To date, family GH139 is the only family known to be able to degrade α1,2-linked MeFuc, making it essential for RG-II metabolism and a feature of RG-II-degrading bacteria. In this report, we present the 3D structure of BT0984GH139, alongside its homolog SDT91673.1GH139 from Verrucomicrobium sp. GAS474, an organism isolated from forest soil. Crystals of BT0984GH139 formed in space group P212121 and diffracted to a resolution of 2.7 Å, while crystals of SDT91673.1GH139 formed in space group P 6522 and diffracted to 2.05 Å, providing good quality electron density maps in both cases. Both proteins adopt a three-domain architecture, consisting of an N-terminal β-sheet domain leading into an α-helical domain composed of a core (α/α)6 toroid structure. GH139 enzymes operate via an inverting mechanism in which we propose that N412 functions as the catalytic base and E561 acts as the catalytic acid (BT0984GH139 numbering).

The B. theta protein BT0984 was the founding member of GH139 (BT0984GH139) and is specific for the α1,2-linked MeFuc in chain B(6). BT0984GH139 specifically cleaves α1,2 linked MeFuc in partially digested RG-II but cannot access this residue within the intact polysaccharide. However, once the preceding arabinofuranose (Araf) and rhamnose (Rha) residues have been removed, BT0984GH139 can efficiently remove MeFuc from isolated chain B. BT0984GH139 exhibited no activity on 4-nitrophenyl α-L-fucoside (4NP-Fuc) but displayed activity on 4-nitrophenyl 2-O-methyl-α-L-fucoside (4NP-MeFuc). By 3 h the anomeric signals had reached equilibrium. These data indicate BT0984GH139 produces β-MeFuc and performs cleavage with inversion of the anomeric configuration of the α-MeFuc linkage. In BT0984GH139, a triad of Trp residues, W162, W403, and W490, lines the putative positively numbered subsites, providing aromatic stacking interactions for sugars within the Δbt0984 oligo. D723 forms hydrogen bonds with both N412 and N729, at distances of 3.3 Å and 2.9 Å, respectively, suggesting it may fulfill the role of activating N412 to function as a catalytic base. In BT0984GH139, the amide side chain of Q411 is positioned 3.5 Å from the catalytic acid E561, and could fulfill the same role as N421 in AfcAGH95 upon substrate binding. Surprisingly, overnight endpoint assays revealed that only one mutation in BT0984GH139, E561A, completely inactivated the enzyme. Based on these data, and with comparison to GH95, it appears that N412 and E561 function as the catalytic base and acid, respectively, in an inverting catalytic mechanism.

>[2x]MGSSHHHHHHSSGPQQGLRQHANVVWDTPSRNSSESMPCGGGDIGMNIWVEEGDILFYLSRSGTFDENNCQLKQGRFRLRLSPNPFEDAKDFRQELKLIDGYVEISAEGTQVQLWADVFHPVVHIEVINDRPLQAEIFYENWRYQDRLIRKGEGQQCSYKWAPPKGTMTHADFISLENSSEKDSKRLLFYHRNAEETVFDVAVAQQGMNEVKSQMMNPLKNLTFGGYLSGENLEYIGTSDSVYAGTDYRAWGFRSLKASKKHHFSVVLHTEQTETVTQWEQGLKTAWQRIAPQGKISSKVVSQDKKQTRLWWNAFWQRSFIETIGETENKENSKVEKETGNKEKSDAKDALKEITRNYTLFRYMLGCNAYGSVPTKFNGGLFTFDPCHIDEKQAFTPDYRKWGGGTMTAQNQRLVYWPMLKSGDFDMMPSQFNFYNRMLKNAELRSHVYWQHEGACFCEQIENFGLPNPAEYGFKRPAWFDKGLEYNAWLEYEWDTILEFCQMILETKNYAGADITPYLPLIESSLTFFDEHYRLLASRRGRKALDGDGHLILFPGSACETYKMTNNASSTIAALRTVLETYIKVCNNEKWQKMLETIPPVPLRYIEVKDSLNLQASTMTPAWKQTISPAKSWERINNIETPQLYPVFPWRIYGVGKENLEIARDTYFYDPDALKFRSHTGWKQDNIWAACLGLTEEAKSLSLAKLSDGPHRFPAFWGPGYDWTPDHNWGGSGMIGLQEMLLQTNGTQILLFPAWPKEWNVHFKLHAPGNTTVEATLKDGKVTILKVSPESRKKDIVIMIEK> MSSYVDKLDITQKQLRFLHKQFKEIIDEKVRTALPESSEDDQVSQEIQLQLDQFLMDVLEMAGESMNVVDAGKGTTVKSVIQEVQKEYTEPFDVELNEKVRKLYQEWEDETVKVSKLRRE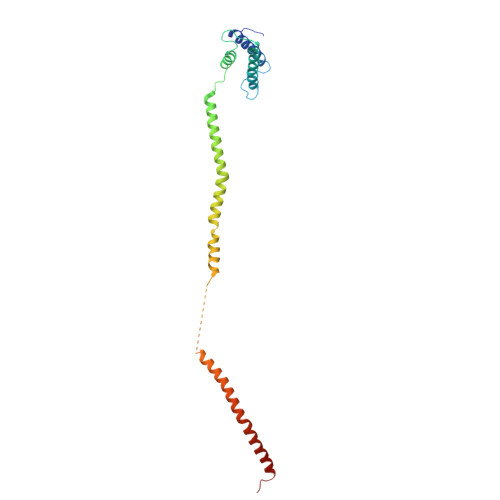APQVAVSEYTKQENQLLEEIDSLIAKMDSSQPNLQNEDQDEGQNEEKTQEYWNQVANQYGSILTSLKEINDKIPTHESKQKRLRLLLDLIEKEVAT>[2x]TALAEMPKRKFTIDDFDIGRPLGKGKFGNVYLAREKQNKFIMALKVLFKSQLEKEG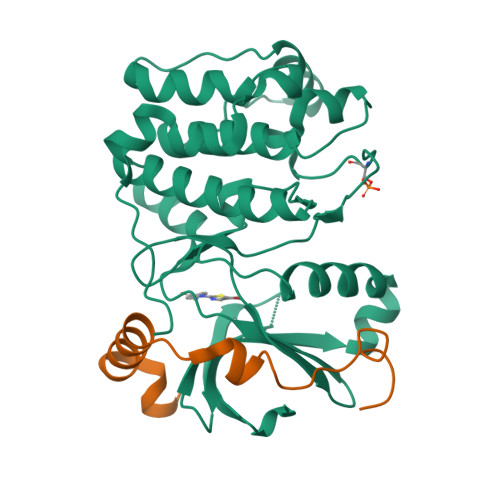VEHQLRREIEIQSHLRHPNILRMYNYFHDRKRIYLMLEFAPRGELYKELQKHGRFDEQRSATFMEELADALHYCHERKVIHRDIKPENLLMGYKGELKIADFGWSVHAPSLRRRTMCGTLDYLPPEMIEGKTHDEKVDLWCAGVLCYEFLVGMPPFDSPSHTETHRRIVNVDLKFPPFLSDGSKDLISKLLRYHPPQRLPLKGVMEHPWVKANSRRVLPPVYQSTQSK;>IPAWASGNLLTQAIRQQYYKPIDVDRMYGTIDSPKLEELFNKS[2x]>MATLATKKATLVAALKDLQRVTVAFSGGIDSTLVLKMALDVLGRDNVTAVVANSELFTDEEFDKAMSLAEELGANVQGTTLDYLSDDHIKNNTPDSWYYAKKMFYSRLNDIAANNGSAAVLDGMIKNDENDYRPGLKARSEAGARSLLQEADFFKTDVRALAQELGL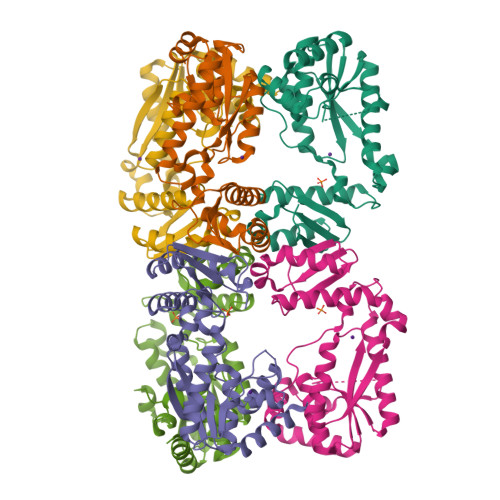TNWNKVASCSVSSRFPYGTTLTHDNIAQVMAAEKYLRSLGFPTVRVRFHNDIARIELPEARIGDFLVFNDRVNRQLQSLGFRYVTLDLGGFRSGRMNDTLTKAQLATFAASWSHPQFEK[12x]(6P)-2-{(3S)-1-[(2-methoxypyrimidin-5-yl)methyl]piperidin-3-yl}-6-(thiophen-2-yl)pyrimidin-4-ol | C19 H21 N5 O2 S 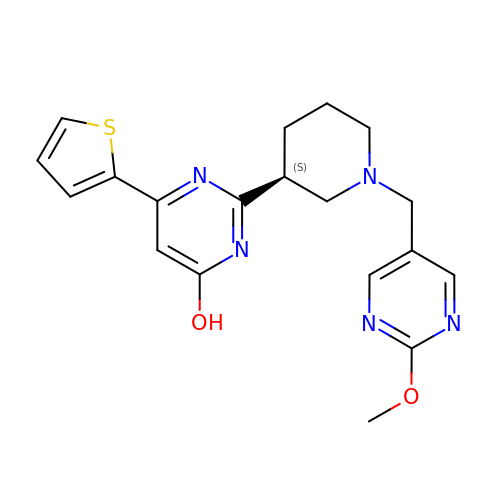| NVEPPHORIAFPBH-AWEZNQCLSA-N> MTGPTRALFLSSGINLGRLRLAEQFSSMNGWQSKEDPAFDAYVKERRRKENYEAFDQRVERGYAAAAKLHKAEIQNAVKRRLKSSGAKFTAETLREMSSAVTERLAWLRDVWAQIDADYRSGDSARQETAAQEISAALRGEPNDYMRWVYETKRELRFAGPVGRRAIQEELQAAELPEVLDEEVNRYHDLKLNMMEIEREVKAKYGVAGQQHWAELQAAKDEEYIQKLDEAAEVYKQLLDQSARLDESRRSELQRSYVERVHQAQVRFKAAMELEGQREQLIEAHQAMKEERMRTEREKRRQLLREA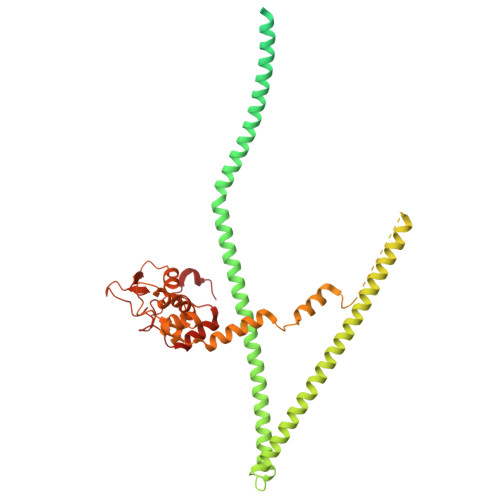AELRAQGKKSADVLTALKERQLDANAKRQAEYELKECEDILKRKSEMLDMIAHFKHDVEEREGREMLQRQKSDEERQVNVFGFYEEVGVEDGLSISSEGTTSQGGSSGLGTVSTSTSCAKSADSNSSAQPSQKLRKEELWKVINADTYEDPFRTVHQARLDAVKTYDPAYARTFPLNLVLGRKYSRQGAGEMAAGNETDKQILQKGNNILYSFQWGLNNGTVHDLDADGGTDYFMDGAFHVRDKETGDIDWRYEKKRGGPVFRGPKFYRLGAQREAADPGERAMDPTPYTSTPREHKWRSS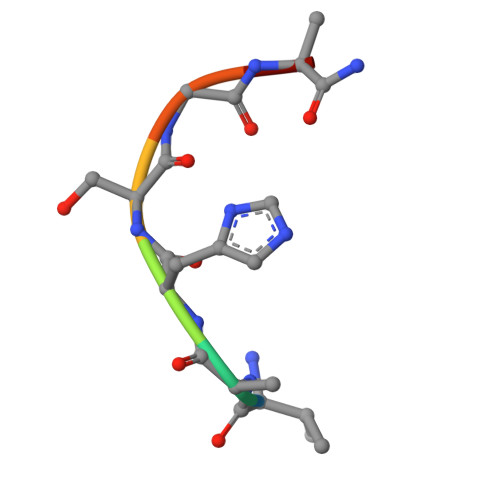> VAHSGAK> MEKQWWKESVVYQIYPRSFMDSNGDGIGDLRGIISKLDYLKELGIDVIWLSPVYESPNDDNGYDISDYCKIMNEFGTMEDWDELLHEMHERNMKLMMDLVVNHTSDEHNWFIESRKSKDNKYRDYYIWRPGKEGKEPNNW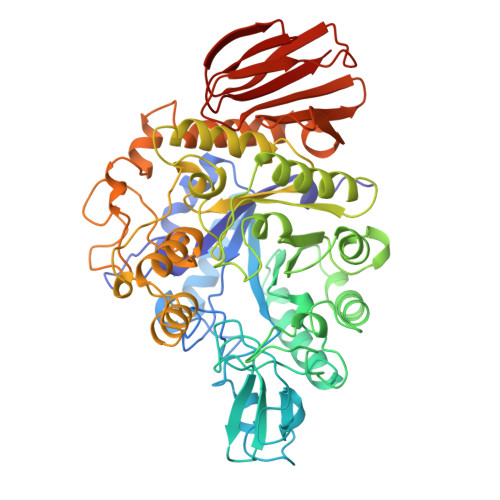GAAFSGSAWQYDEMTDEYYLHLFSKKQPDLNWDNEKVRQDVYEMMKFWLEKGIDGFRMDVINFISKEEGLPTVETEEEGYVSGHKHFMNGPNIHKYLHEMNEEVLSHYDIMTVGEMPGVTTEEAKLYTGEERKELQMVFQFEHMDLDSGEGGKWDVKPCSLLTLKENLTKWQKALEHTGWNSLYWNNHDQPRVVSRFGNDGMYRIESAKMLATVLHMMKGTPYIYQGEEIGMTNVRFESIDEYRDIETLNMYKEKVMERGEDIEKVMQSIYIKGRDNARTPMQWDDQNHAGFTTGEPWITVNPNYKEINVKQAIQNKDSIFYYYKKLIELRKNNEIVVYGSYDLILENNPSIFAYVRTYGVEKLLVIANFTAEECIFELPEDISYSEVELLIHNYDVENGPIENITLRPYEAMVFKLK>GGACUAGUCC[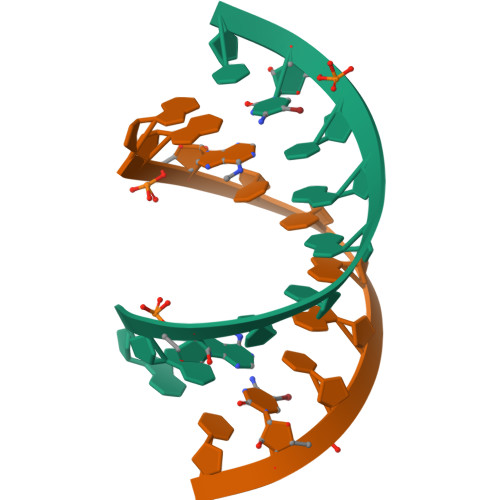4x]>MRGSHHHHHHGSMNPAAEAEFNILLATDSYKVTHYKQYPPNTSKVYSYFECREVKYEETVFYGLQYILNKYLKGKVVTKEKIQEAKDVYKEHFQDDVFNEKGWNYILEKYDGHLPIEIKAVPEGFVIPRGNVLFTVENTDPECYWLTNWIETILVQSWYPITVATNSREQKKILAKYLLETSGNLDGLEYKLHDFGYRGVSSQETAGIGASAHLVNFKGTDTVAGLALIKKYYGTKDPVPGYSVPAAEHSTITAWGKDHEKDAFEHIVTQFSSVPVSVVSDSYDIYNACEKIWGEDLRHLIVSRSTQAPLIIRPDSGNPLDTVLKVLEILGKKFPVTENSKGYKLLPPYLRVIQGDGVDINTLQEIVEGMKQKMWSIENIAFGSGGGLLQKLTRDL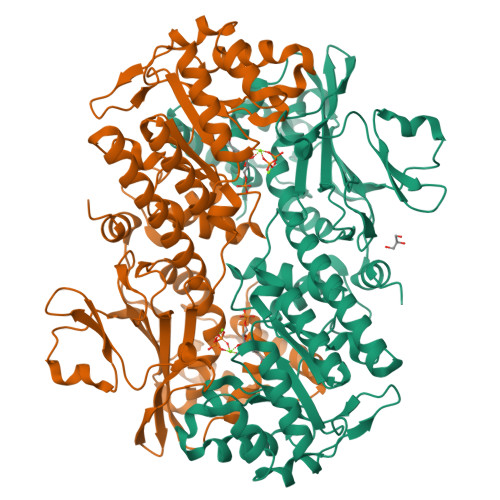LNCSFKCSYVVTNGLGINVFKDPVADPNKRSKKGRLSLHRTPAGNFVTLEEGKGDLEEYGQDLLHTVFKNGKVTKSYSFDEIRKNAQLNIELEAAHH[2x]>MVHYRTIDSPIGPLTLAGHGSVLTNLRMLEQTYEPSRTHWTPDPGAFSGAVDQLNAYFAGELTEFDVELDLRGTDFQQRVWKALLTIPYGETRSYGEIADQIGAPGAARAVGLANGHNPIAIIVPCHRVIGASGKLTGYGGGINRKRALLELE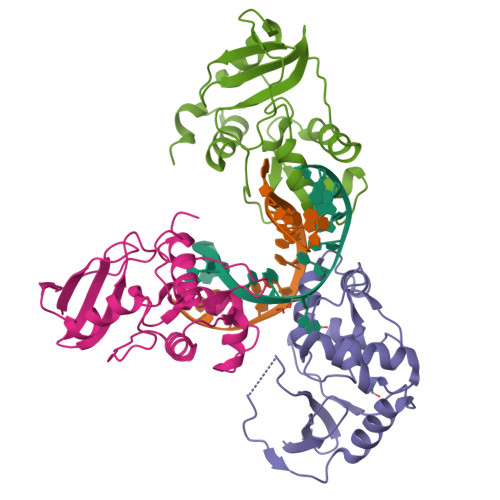KSRAPADLTLFD[3x]>SMPKLPENYTDETWQKLKEAVEAIQNSTSIKYNLEELYQAVENLCSYKISANLYKQLRQICEDHIKAQIHQFREDSLDSVLFLKKIDRCWQNHCRQMIMIRSIFLFLDRTYVLQNSMLPSIWDMGLELFRAHIISDQKVQNKTIDGILLLIERERNGEAIDRSLLRSLLSMLSDLQIYQDSFEQRFLEETNRLYAAEGQKLMQEREVPEYLHHVNKRLEEEADRLITYLDQTTQKSLIATVEKQLLGEHLTAILQKGLNNLLDENRIQDLSLLYQLFSRVRGGVQVLLQQWIEYIKAFGSTIVINPEKDKTMR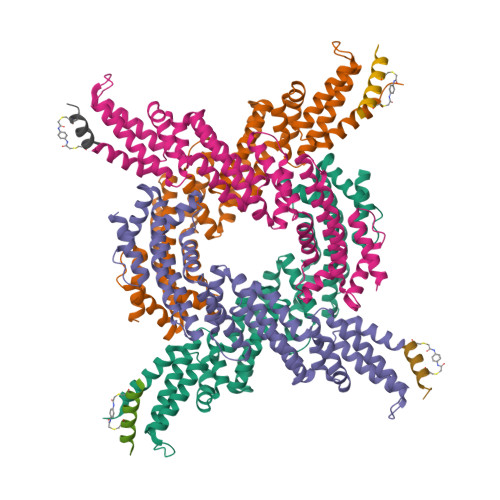QELDDFKDKVDHIIDICFLKNEKFINAMKEAFETFINKRPN[4x];>[4x]XDPADRWCELAAWTCDTFX N'-Formylkynurenine 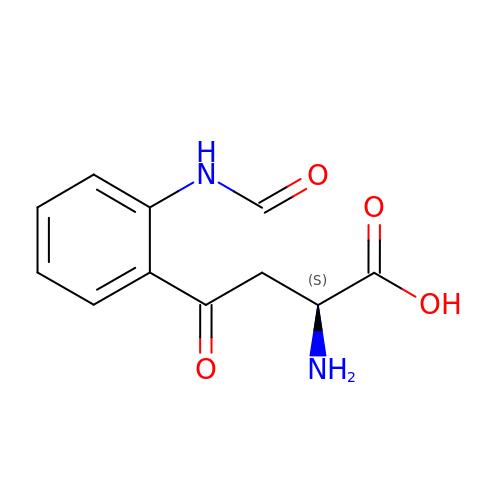| C11 H12 N2 O4 | BYHJHXPTQMMKCA-QMMMGPOBSA-N> MEVKELERDKNRVVLEYVFGAEEIAQAEDKAVRYLNQRVEIPGFRKGRIPKNVLKMKLGEEFQEYTLDFLMDLIPDTLKDRKLILSPIVTERELKDVTARVVVEVHEEPEVRIGDISKIEVEKVDEEKVLEKYVERRIEDLRESHALLEPKEGPAEAGDLVRVNMEVYNEEGKKLTSREYEYVISEDEDRPFVKDLVGKKKGDVVEIEREYEGKKYTYKLEVEEVYKRTLPEIGDELAKSVNNEFETLEQLKESLKKEGKEIYDVEMKESMREQLLEKLPEIVEIEISDRTLEILVNEAINRLKREGRYEQIVSSYESEEKFREELKERILDDIKRDRVIEVLAQEKGISVNDEELEKEAEELAPFWGISPDRAKS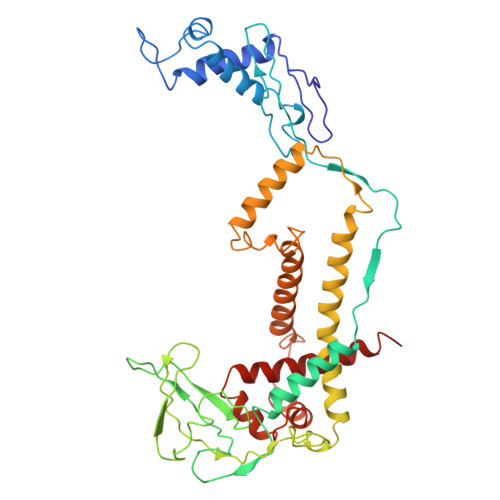LVKARQDLREELRWAILKRKVLDLLLQEVE>[4x]MWSHPQFEKGSGSENLYFQGTMKVINDPIHGHIELHPLLVRIIDTPQFQRLRYIKQLGGGYYVFPGASHNRFEHSLGVGYLAGCLVHALGEKQPELQISERDVLCVQIAGLCHDLGHGPFSHMFDGRFIPLARPEVKWTHEQGSVMMFEHLINSNGIKPVMEQYGLIPEEDICFIKEQIVGPLESPVEDSLWPYKGRPENKSFLYEIVSNKRNGIDVAKWDYFARDCHHLGIQNNFDYKRFIKFARVCEVDNELRICARDKEVGNLYDMFHTRNSLHRRAYQHKVGNIIDTMITDAFLKADDYIEITGAGGKKYRISTAIDDMEAYTKLTDNIFLEILYSTDPKLKDAREILKQIEYRNLFKYVGETQPTGQIKIKREDYESLPKEVASAKPKVLLDVKLKAEDFIVDVINMDYGMQEKNPIDHVSFYCKTAPNRAIRITKNQVSQLLPEKFAEQLIRVYCKKVDRKSLYAARQYFVQWCADRNFTKPQDGDVIAPLITPQKKEWNDSTSVQNPTRLREASKSRVQLFKDDPM

Identification of SAMHD1 as the factor that impedes infection of myeloid cells by HIV and SIV brought to light an intrinsic cellular antiviral immunity mechanism that relies on controlled reduction of deoxynucleotide triphosphate (dNTP) availability. To counter this infectivity block, HIV-2 and SIV viruses encode an auxiliary protein Vpx, which targets SAMHD1 for proteasomal degradation and facilitates infection of noncycling immune cells by these viruses. In this study, we show that the allosteric binding sites of the enzyme are plastic and can accommodate oligonucleotides in place of the allosteric activators, GTP and dNTP. Collectively, our results shed new light onto the intricate allosteric regulation of SAMHD1 activity and raise questions about the role of nucleic acid phosphorothioation in dNTP metabolism and antiviral immunity in bacteria and in humans.

To gain further mechanistic insight into the interaction of SAMHD1 with nucleic acids, we determined structures of SAMHD1114–626 bound to the phosphorothioate-linked deoxy(C*G*C*C*T) and the phosphodiester-linked ribo(CGCCU) oligonucleotides by X-ray crystallography. In contrast, in our oligonucleotide-bound structures, only the dimer-1 interface is intact, but the packing of the two SAMHD1 dimers in the asymmetric unit is looser, the dimer-2 (tetramer) interface is not properly formed, and no 222-point symmetry is present. We conclude that in our crystals, the content of the asymmetric unit represents crystal packing of two oligonucleotide-bound SAMHD1 dimers. The structures revealed that bound oligonucleotides span both allosteric binding sites A1 and A2 and engage many of the same residues that mediate binding of nucleotide triphosphates. For example, the guanine nucleobase of the sole G nucleotide within the oligos is accommodated in the guanine-recognition pocket of the A1 formed by SAMHD1 residues D137, Q142, R145, and R451. The key difference between the oligonucleotide-bound and nucleotide-triphosphate-bound structures is that in the nucleotide-triphosphate-bound tetramer, the allosteric ligands in the A1 and A2 sites make contacts with residues of three distinct monomers, whereas in our oligonucleotide-bound structures, residues of only two monomers are involved. The structures also offer insight into why phosphorothioation increases oligonucleotide-binding affinity. In the d(C*G*C*C*T)-bound structure, histidine H376 appears to form a hydrogen bond with one of the nonbridging atoms of the phosphorothioate linkage between the G2 and C3 nucleotides in the oligo. A similar contact is observed between H125 and the phosphorothioate bond between C3 and C4. Although the resolution of the electron-density map limited our ability to determine positions of sulfur atoms in the phosphorothioate linkages in the d(C*G*C*C*T)-SAMHD1 complex with high confidence, the data indicated that the interaction may be stereoselective.>[2x]GSVAGRIVIDDVQPVVSNGRYPAKAVVGEVVPVAATVWREGHDAVAATLVVRYHGTTYPDLADPPPGVPGADRTAVPIGDVMTPAAPVKPQRLPMSPGHTPDVFHGHFTPDRVGLWTYRVDGWGDPIASWRHNVTAKLDAGQGESELNNDLLVGARLLERAATGVPRELREALLEAAAALRAPGDPFTRAGAALSAEVSDLLAEYPLREFVTRGEQYGVWVDRPEARFSSWYEMFPRSTGGWDAEGRPVHGTFATAAEALPRIARMGFDVVYLPPIHPIGKVHRKGRNNSVTAAPGDVGSPWAIGSDEGGHDAVHPQLGTIEDFDEFVASARDLGLEVALDLALQCAPDHPWAREHPEWFTVLPDGSIAYAENPPKKYQDIYPLNFDNDPAGIYQEVLRVVRFWISHGVNIFRVDNPHTKPPNFWAWLIGQIKNENPDVLFLSEAFTRPARLYGLAKLGFTQSYTYFTWRTSKWELTEFGQEIAAKADIARPNLFVNTPDILHESLQHGGPGMFAIRAVLAATMGPAWGVYSGYELFENQPVRPGSEEYLNSEKYELRPRDFESALARGESLEPFLTRLNEIRRLHPALRELRTIRFHHVDNDALLAYSKFDPGTGDTVLVVVTLNPFGAEEATLWLDMPELGMEPYDRFWVRDEITGEEYQWGQANYVRLDPAKAVAHVLNMPLIPADKRLQLLRRE

GlgE is a maltosyl transferase that transfers maltose from a maltose-1-phosphate (maltose-1P) donor to α-(1–4) glucan chains. GlgE is essential for M. tuberculosis and its depletion leads to pleiotropic stress effects and eventually cell death. GlgE is proposed to catalyse the transfer of maltosyl units to α-glucan chains through a double-displacement reaction in which an aspartate residue acts as a nucleophile forming an β-maltosyl-enzyme intermediate, while a glutamate residue is thought to protonate the phosphate and deprotonate the acceptor, acting like an acid/base catalytic residue16. Each of the protomers of M. thermoresistibile GlgE contains 5 domains and 2 inserts that have been described extensively in the first reported GlgE structure and therefore we will focus on the particular characteristics of M. thermoresistibile GlgE.

However, we could only obtain high-resolution crystals (~2.0 Å) when GlgE was co-crystalized with maltose, maltohexaose or both. The maltohexaose and maltose co-crystallizations produced indistinguishable structures in which only maltose could be observed at the active site. The structure of M. thermoresistible GlgE was solved by molecular replacement at 1.96 Å and refined with a final R-factor of 0.175 and Rfree of 0.203. From the maltose-bound structure, which is the highest resolution structure reported in this work, we can see that the donor substrate forms hydrogen bonds with the side chains of the highly conserved K283, N287 and S298 of the insert 1. K283 forms hydrogen bonds with the C3 and C4 hydroxyl groups and N287 with C2 hydroxyl group, all from the non-reducing glucose. The donor substrate further interacts with the side chains of the absolutely conserved Q343 and D378 of domain B, R411, D413, E442 and D498 of domain A and K552 and Y553 of insert 2. Two phosphate groups can also be seen bound to each of the chains sitting in a groove between domain N and the terminal α-helix of C. Two other phosphate groups sit in a positively charged patch formed by domains A and N of the two opposing protomers, near the active site. Interestingly all the phosphate groups are close to threonines, T98 for the first duo and T445 for the second. One of the threonines, T445 of domain A, sits close to the active site and within what could be the binding region of the acceptor substrate. This threonine is highly conserved in all mycobacteria species and even in closely related organisms.> MPYIEKL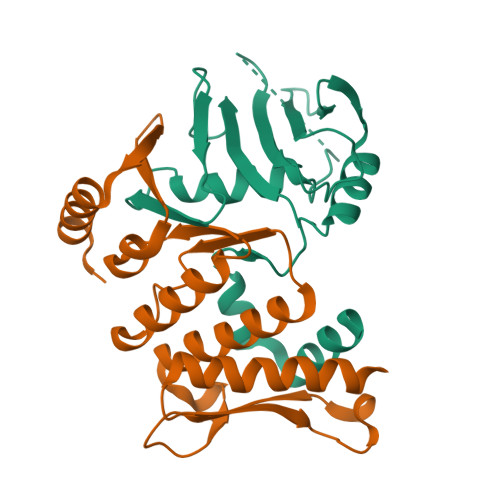ELKGFKSYGNKKVVIPFSKGFTAIVGANGSGKSNIGDAILFVLGGLSAKAMRASRISDLIFAGSKNEPPAKYAEVAIYFNNEDRGFPIDEDEVVIRRRVYPDGRSSYWLNGRRATRSEILDILTAAMISPDGYNIVLQGDITKFIKMSPLERRLLIDDISGIAEYDSKKEKALEE;> EKEKKNVFMRTFEAISRNFSEIFAKLSPGGSARLILENPEDPFSGGLEIEAKPAGKDVKRIEAMSGGEKALTALAFVFAIQKFKPAPFYLFDEIDAHLDDANVKRVADLIKESSKESQFIVITLRDVMMANADKIIGVSMRDGVSKVVSLSLEKAMKILEEIRKKQGWEHGN> MAPLGPTGPLPQSFLLKCLEQMRK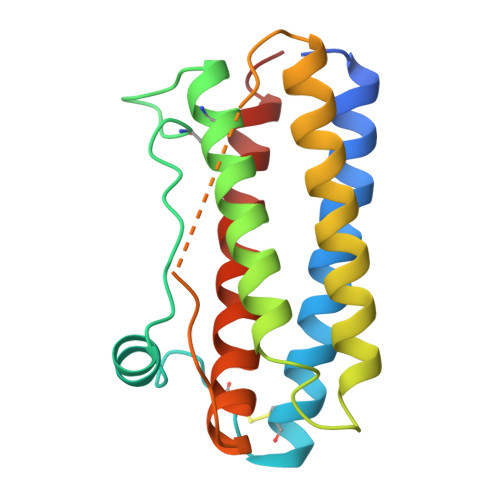VQADGTALQETLCATHQLCHPEELVLLGHALGIPQPPLSSCSSQALQLMGCLRQLHSGLFLYQGLLQALAGISPELAPTLDTLQLDTTDFAINIWQQMEDLGMAPAVPPTQGTMPAFTSAFQRRAGGVLVASNLQSFLELAYRALRHFAKP>[12x]MPTLPKAEAKELSAFVQSCVEYKTNVCFTDVAAYESNQKGVLSSGLAVLVGTHKQLRDPAVQRLPFYNPAVAEAIERVKEGGTYGVLVEGLANAAGSKFVRVVVGEVPTKASRNNCPARPDVVTALVTAALDEVKEPNTTVDVFVLSNAVLPIAAAVARCGKHNFSAKDGAAAAAYNSGKVSRLQVVFPEPPAIPPKDLEAVATSTQLCQRLVDAPPNLLTTATFTEIAQGYAKALGFDVDVICGDDLCERGYGGIYSVGKAAFEAPRLVTLLYTPKGTPVKKVSLVGKGIVYDCGGLALKPADYMKLMKHDMGGAAAVFCGFLTAVRLQQPVQLSCTLCLAENAIGPKSYRNDDIIVMKSGKTVEVINTDAEGRIVLGDGVFHATNELSFTPDVVIDMATLTGAQGIATGRHHAGLYVNEEGAEAAMLRAGRESGETCFPVLYCPEYHEPEFKSNHADMTNLMERRDN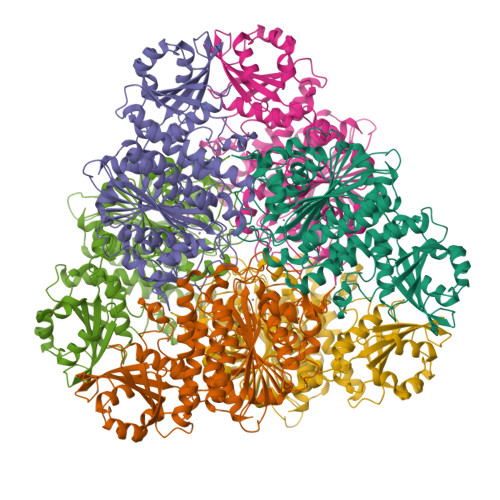AGVSCAGYFITTHLSPKFTGAHIHVDLAYPVFNSNGATGFGPALLTEYFRKL>[4x]GPMDTPENVLQMLEAHMQSYKGNDPLGEWERYIQWVEENFPENKEYLITLLEHLMKEF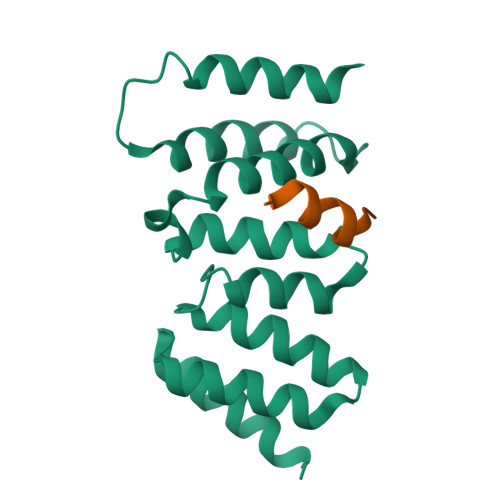LDKKKYHNDPRFISYCLKFAEYNSDLHQFFEFLYNHGIGTLSSPLYIAWAGHLEAQGELQHASAVLQRGIQNQAEPREFLQQQYRLFQTRLTET;>GPQMDLTSSHTVMITKGLLDNPISEKSTKIDTTSFLANLKLHTEDSRMKKEVN[4x]>MAASGLDHLKNGYRRRFCRPSRARDINTEQGQNVLEILQDCFEEKSLANDFSTNSTKSVPNSTRKIKDTCIQSPSKECQKSHPKSVPVSSKKKEASLQFVVEPSEATNRSVQAHEVHQKILATDVSSKNTPDSKKISSRNINDHHSEADEEFYLSVGSPSVLLDAKTSVSQNVIPSSAQKRETYTFENSVNMLPSSTEVSVKTKKRLNFDDKVMLKKIEIDNKVSDEEDKTSEGQERKPSGSSQNRIRDSEYEIQRQAKKSFSTLFLETVKRKSESSPIVRHAATAPPHSCPPDDTKLIEDEFIIDESDQSFASRSWITIPRKAGSLKQRTISPAESTALLQGRKSREKHHNILPKTLANDKHSHKPHPVETSQPSDKTVLDTSYALIGETVNNYRSTKYEMYSKNAEKPSRSKRTIKQKQRRKFMAKPAEEQLDVGQSKDENIHTSHITQDEFQRNSDRNMEEHEEMGNDCVSKKQMPPVGSKKSSTRKDKEESKKKRFSSESKNKLVPEEVTSTVTKSRRISRRPSDWWVVKSEESPVYSNSSVRNELPMHHNSSRKSTKKTNQSSKNIRKKTIPLKRQKTATKGNQRVQKFLNAEGSGGIVGHDEISRCSLSEPLESDEADLAKKKNLDCSRSTRSSKNEDNIMTAQNVPLKPQTSGYTCNIPTESNLDSGEHKTSVLEESGPSRLNNNYLMSGKNDVDDEEVHGSSDDSKQSKVIPKNRIHHKLVLPSNTPNVRRTKRTRLKPLEYWRGERIDYQGRPSGGFVISGVLSPDTISSKRKAKENIGKVNKKSNKKRICLDNDERKTNLMVNLGIPLGDPLQPTRVKDPETREIILMDLVRPQDTYQFFVKHGELKVYKTLDTPFFSTGKLILGPQEEKGKQHVGQDILVFYVNFGDLLCTLHETPYILSTGDSFYVPSGNYYNIKNLRNEESVLLFTQIKR[2x];> MEEQPQMQDADEPADSGGEGRAGGPPQVAGAQAACSEDRMTLLLRLRAQTKQQLLEYKSMVDASEEKTPEQIMQEKQIEAKIEDLENEIEEVKVAFEIKKLALDRMRLSTALKKNLEKISRQSSVLMDNMKHLLELNKLIMKSQQESWDLEEKLLDIRKKRLQLKQASESKLLEIQTEKNKQKIDLDSMENSERIKIIRQNLQMEIKITTVIQHVFQNLILGSKVNWAEDPALKEIVLQLEKNVDMMHHHHHH;> MSPQKRVKNVQAQNRTSQGSSSFQTTLSAWKVKQDPSNSKNISKHGQNNPVGDYEHADDQAEEDALQMAVGYFEKGPIKASQNKDKTLEKHLKTVENVAWKNGLASEEIDILLNIALSGKFGNAVNTRILKCMIPATVISEDSVVKAVSWLCVGKCSGSTKVLFYRWLVAMFDFIDRKEQINLLYGFFFASLQDDALCPYVCHLLYLLTKKENVKPFRVRKLLDLQAKMGMQPHLQALLSLYKFFAPALISVSLPVRKKIYFKNSENLWKTALLAVKQRNRGPSPEPLKLMLGPANVRPLKRKWNSLSVIPVLNSSSYTKECGKKEMSLSDCLNRSGSFPLEQLQSFPQLLQNIHCLELPSQMGSVLNNSLLLHYINCVRDEPVLLRFYYWLSQTLQEECIWYKVNNYEHGKEFTNFLDTIIRAECFLQEGFYSCEAFLYKSLPLWDGLCCRSQFLQLVSWIPFSSFSEVKPLLFDHLAQLFFTSTIYFKCSVLQSLKELLQNWLLWLSMDIHMKPVTNSPLETTLGGSMNSVSKLIHYVGWLSTTAMRLESNNTFLLHFILDFYEKVCDIYINYNLPLVVLFPPGIFYSALLSLDTSILNQLCFIMHRYRKNLTAAKKNELVQKTKSEFNFSSKTYQEFNHYLTSMVGCLWTSKPFGKGIYIDPEILEKTGVAEYKNSLNVVHHPSFLSYAVSFLLQESPEERTVNVSSIRGKKWSWYLDYLFSQGLQGLKLFIRSSVHHSSIPRAEGINCNNQY;> MNQEDLDPDSTTDVGDVTNTEEELIRECEEMWKDMEECQNKLSLIGTETLTDSNAQLSLLIMQVKCLTAELSQWQKKTPETIPLTEDVLITLGKEEFQKLRQDLEMVLSTKESKNEKLKEDLEREQRWLDEQQQIMESLNVLHSELKNKVETFSESRIFNELKTKMLNIKEYKEKLLSTLGEFLEDHFPLPDRSVKKKKKNIQESSVNLITLHEMLEILINRLFDVPHDPYVKISDSFWPPYVELLLRNGIALRHPEDPTRIRLEAFHQ;> MDSYSAPESTPSASSRPEDYFIGATPLQKRLESVRKQSSFILTPPRRKIPQCSQLQEDVDPQKVAFLLHKQWTLYSLTPLYKFSYSNLKEYSRLLNAFIVAEKQKGLAVEVGEDFNIKVIFSTLLGMKGTQRDPEAFLVQIVSKSQLPSENREGKVLWTGWFCCVFGDSLLETVSEDFTCLPLFLANGAESNTAIIGTWFQKTFDCYFSPLAINAFNLSWMAAMWTACKMDHYVATTEFLWSVPCSPQSLDISFAIHPEDAKALWDSVHKTPGEVTQEEVDLFMDCLYSHFHRHFKIHLSATRLVRVSTSVASAHTDGKIKILCHKYLIGVLAYLTELAIFQIE;> MSVLRPLDKLPGLNTATILLVGTEDALLQQLADSMLKEDCASELKVHLAKSLPLPSSVNRPRIDLIVFVVNLHSKYSLQNTEESLRHVDASFFLGKVCFLATGAGRESHCSIHRHTVVKLAHTYQSPLLYCDLEVEGFRATMAQRLVRVLQICAGHVPGVSALNLLSLLRSSEGPSLEDL;> MDETVAEFIKRTILKIPMNELTTILKAWDFLSENQLQTVNFRQRKESVVQHLIHLCEEKRASISDAALLDIIYMQFHQHQKVWEVFQMSKGPGEDVDLFDMKQFKNSFKKILQRALKNVTVSFRETEENAVWIRIAWGTQYTKPNQYKPTYVVYYSQTPYAFTSSSMLRRNTPLLGQALTIASKHHQIVKMDLRSRYLDSLKAIVFKQYNQTFETHNSTTPLQERSLGLDINMDSRIIHENIVEKERVQRITQETFGDYPQPQLEFAQYKLETKFKSGLNGSILAEREEPLRCLIKFSSPHLLEALKSLAPAGIADAPLSPLLTCIPNKRMNYFKIRDKHHHHHH;>MEQANPLRPDGESKGGVLAHLERLETQVSRSRKQSEELQSVQAQEGALGTKIHKLRRLRDELRAVVRHRRASVKACIANVEPNQTVEINEQEALEEKLENVKAILQAYHFTGLSGKLTSRGVCVCISTAFEGNLLDSYFVDLVIQKPLRIHHHSVPVFIPLEEIAAKYLQTNIQHFLFSLCEYLNAYSGRKYQADRLQSDFAALLTGPLQRNPLCNLLSFTYKLDPGGQSFPFCARLLYKDLTATLPTDVTVTCQGVEVLSTSWEEQRASHETLFCTKPLHQVFASFTRKGEKLDMSLVS[2x];> MDAELAEVRALQAEIAALRRACEDPPAPWEEKSRVQKSFQAIHQFNLEGWKSSKDLKNQLGHLESELSFLSTLTGINIRNHSKQTEDLTSTEMTEKSIRKVLQRHRLSGNCHMVTFQLEFQILEIQNKERLSSAVTDLNIIMEPTECSELSEFVSRAEERKDLFMFFRSLHFFVEWFEYRKRTFKHLKEKYPDAVYLSEGPSSCSMGIRSASRPGFELVIVWRIQIDEDGKVFPKLDLLTKVPQRALELDKNRAIETAPLSFRTLVGLLGIEAALESLIKSLCAEENN;> MSGKANASKKNAQQLKRNPKRKKDNEEVVLSENKVRNTVKKNKNHLKDLSSEGQTKHTNLKHGKTAASKRKTWQPLSKSTRDHLQTMMESVIMTILSNSIKEKEEIQYHLNFLKKRLLQQCETLKVPPKKMEDLTNVSSLLNMERARDKANEEGLALLQEEIDKMVETTELMTGNIQSLKNKIQILASEVEEEEERVKQMHQINSSGVLSLPELSQKTLKAPTLQKEILALIPNQNALLKDLDILHNSSQMKSMSTFIEEAYKKLDASHHHHHH;> MPVKRSLKLDGLLEENSFDPSKITRKKSVITYSPTTGTCQMSLFASPTSSEEQKHRNGLSNEKRKKLNHPSLTESKESTTKDNDEFMMLLSKVEKLSEEIMEIMQNLSSIQALEGSRELENLIGISCASHFLKREMQKTKELMTKVNKQKLFEKSTGLPHKASRHLDSYEFLKAILN;> MEEEAETEEQQRFSYQQRLKAAVHYTVGCLCEEVALDKEMQFSKQTIAAISELTFRQCENFAKDLEMFARHAKRTTINTEDVKLLARRSNSLLKYITDKSEEIAQINLERKAQKKKKSEDGSKNSRQPAEAGVVESEN;> MADHNPDSDSTPRTLLRRVLDTADPRTPRRPRSARAGARRALLETASPRKLSGQTRTIARGRSHGARSVGRSAHIQASGHLEEQTPRTLLKNILLTAPESSILMPESVVKPVPAPQAVQPSRQESSCGSLELQLPELEPPTTLAPGLLAPGRRKQRLRLSVFQQGVDQGLSLSQEPQGNADASSLTRSLNLTFATPLQPQSVQRPGLARRPPARRAVDVGAFLRDLRDTSLAPPNIVLEDTQPFSQPMVGSPNVYHSLPCTPHTGAEDAEQAAGRKTQSSGPGLQKNSPGKPAQFLAGEAEEVNAFALGFLSTSSGVSGEDEVEPLHDGVEEAEKKMEEEGVSVSEMEATGAQGPSRVEEAEGHTEVTEAEGSQGTAEADGPGASSGDEDASGRAASPESASSTPESLQARRHHQFLEPAPAPGAAVLSSEPAEPLLVRHPPRPRTTGPRPRQDPHKAGLSHYVKLFSFYAKMPMERKALEMVEKCLDKYFQHLCDDLEVFAAHAGRKTVKPEDLELLMRRQGLVTDQVSLHVLVERHLPLEYRQLLIPCAYSGNSVFPAQ;> MAPRGRRRPRPHRSEGARRSKNTLERTHSMKDKAGQKCKPIDVFDFPDNSDVSSIGRLGENEKDEETYETFDPPLHSTAIYADEEEFSKHCGLSLSSTPPGKEAKRSSDTSGNEASEIESVKISAKKPGRKLRPISDDSESIEESDTRRKVKSAEKISTQRHEVIRTTASSELSEKPAESVTSKKTGPLSAQPSVEKENLAIESQSKTQKKGKISHDKRKKSRSKAIGSDTSDIVHIWCPEGMKTSDIKELNIVLPEFEKTHLEHQQRIESKVCKAAIATFYVNVKEQFIKMLKESQMLTNLKRKNAKMISDIEKKRQRMIEVQDELLRLEPQLKQLQTKYDELKERKSSLRNAAYFLSNLKQLYQDYSDVQAQEPNVKETYDSSSLPALLFKARTLLGAESHLRNINHQLEKLLDQG;> MALSTIVSQRKQIKRKAPRGFLKRVFKRKKPQLRLEKSGDLLVHLNCLLFVHRLAEESRTNACASKCRVINKEHVLAAAKVILKKSRG;> MEGAGAGSGFRKELVSRLLHLHFKDDKTKVSGDALQLMVELLKVFVVEAAVRGVRQAQAEDALRVDVDQLEKVLPQLLLDF

The CENP-A nucleosome (CENP-ANuc) is surrounded by a group of 16 proteins, the constitutive centromere-associated network (CCAN) and organized in various stable subcomplexes. Human CCAN is composed by five modules of CENP-C, CENP-LN, CENP-HIKM, CENP-OPQUR and CENP-TWSX. The arrangement of the four sub-complexes generates a b-shaped structure, in which CENP-OPQUR adopts an elongated shape to generate the arm, and CENP-LN, CENP-HIKM, and CENP-TWSX form the semi-circle. The CENP-LN sub-complex, located at the center of the ‘b’, functions as a node for coordination of the assembly of CCAN by contributing the contact sites, with the sub-complexes CENP-HIKM and CENP-OPQU on the opposite side.

Further classifications and reconstructions gave two maps with distinct features in an interior tunnel, representing the CCAN complex alone (apo-CCAN) and CCAN in complex with a fragment of DNA (CCAN-DNA). The built model was then docked into the EM map of CCAN–DNA complex at 3.7 Å and further refined. The structure of CCAN–DNA complex was built into the cryo-EM map at 3.7 Å resolution in which a DNA double helix about 25 bp in length is clearly resolved. Around the DNA is a positively charged channel composed by CENP-LN, CENP-HIKhead, CENP-TW, which is complement to the negative charge of DNA gyre. CCAN complex binds to double-strand DNA through the electrostatic interaction between a set of positively charged residues from several CCAN components and the negatively charged phosphate backbone of DNA, which supports the previous reports that functional kinetochore assembly is independent of DNA sequence. The duplex DNA is topologically entrapped by human CCAN. In our CCAN–DNA structure, CENP-LN coordinates to form a closed channel with positive charge to encompass a double-strand DNA which is similar to CENP-LN interaction with unwrapped DNA in yeast CCAN-CENP-ANuc. Compared to the structure of S. cerevisiae CCAN-CENP-ANuc complex, both human and yeast CCAN complex bind DNA at the same positively charged grooves assembled by the coordination of CENP-LN sub-complex. However, human CENP-LN has a narrower opening, probably caused by the shorter CENP-NCter which leads to the formation of a more compact conformation of the human CCAN complex further strengthened by the interaction with CENP-M. Therefore, human CCAN adopts a close ‘b’ shaped conformation to grip double strand DNA, while yeast CCAN forms a more open structure to accommodate CENP-ANuc.>MGSSHHHHHHSSGENLYFQGHMSSTFEPATDSPLPVPGVQYFLQHVQSGKYVHPHGGSDMPGNDTALVLHHGFDEKRDALRWVFVNDAENKHQLKHYSSGKFVHPKGGKVGKEATLVVHSSPGRPETMIEMVQEDGRTYLRHTDSDYYVHPHGGSPNPGDNTRLVYYSGYRPSLAFLAIPAETLFVDRIEIHQAQALESINTITSLSDEHRNDTDQPVQTSISVALEESLQDSAQLSFERCFGLKVGSEFEVGLPLVGKTKVSVQFSGSWKSSTIKGEVRTSAVKVQINEHVTIPPGKCVQIRIDTRRCTKTAPATMYLRTASGIEVQRETTVTSTYHYDQEVHVVPVTN[2x]

TrefLec was searched for original domain combinations, which led to single out SaroL-1 in the choanoflagellate Salpingoeca rosetta, that contains both β-trefoil and aerolysin-like pore-forming domains. Recombinant SaroL-1 is shown to bind galactose and derivatives, with a stronger affinity for cancer-related α-galactosylated epitopes such as the glycosphingolipid Gb3, when embedded in giant unilamellar vesicles or cell membranes. SaroL-1 is composed of two domains, a β-trefoil domain at the N-terminal region shown in blue and an elongated domain (green) consisting of seven β-strands forming a twisted β-sheet. The lectin-binding step is necessary for the pore-formation since the pre-incubation with a high affinity galactose derivative diminishes or abolishes hemolysis, GUVs penetration, and cytotoxicity.

Several crystals were obtained, those of the complex SaroL-1/GalNAc and SaroL-1/Gb3 trisaccharide showed suitable diffraction and datasets were collected at 1.7 Å and 1.8 Å, respectively. The overall structure of SaroL-1/GalNAc consists of two monomers in the asymmetric unit. They are highly similar (RMSD = 0.52 Å) and do not present extensive contact, confirming the monomeric state of the lectin in solution. Clear electron density for three GalNAc monosaccharides is observed in the lectin domain, corresponding to the three sites α, β and γ, classically observed in the β-trefoil structure. In all sites, both α- and β-anomers of the GalNAc monosaccharides are present, with stronger occupancy for the α anomer. The axial O4 of αGalNAc establishes hydrogen bonds with the side chain of conserved His and Arg residues in all sites. This Arg also interacts with the O3 hydroxyl establishing fork-like contacts with two adjacent oxygens of the sugar ring. The O6 hydroxyl is hydrogen-bonded to the main chain of a conserved Gly residue and to the side chain oxygen of a more variable Asn/Asp/Glu residue. Moreover, each GalNAc is stabilized in the binding pocket by a C-π-stacking interaction between its hydrophobic face and the aromatic ring of His (site α and β) or Tyr (site γ). The N-acetyl group of GalNAc establishes mostly water-mediated contacts, confirming that it is not crucial for affinity.> MEQCGAQAGGARCPNCLCCSRWGWCGTTSDFCGDGCQSQCSGCGPTPTPTPPSPSDGVGSIVPRDLFERLLLHRNDGACPARGFYTYEAFLAAAAAFPAFGGTGNTETRKREVAAFLGQTSH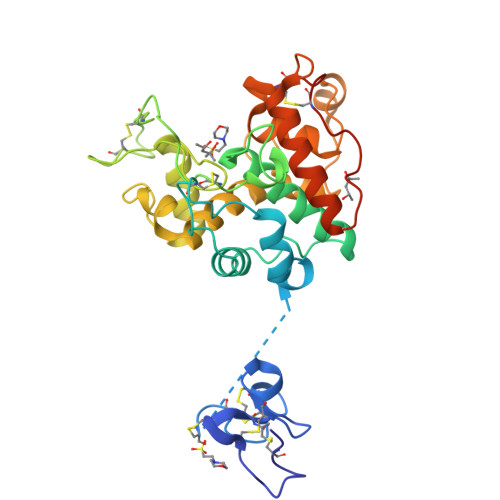ETTGGWPTAPDGPFSWGYCFKQEQNPPSDYCQPSPEWPCAPGRKYYGRGPIQLSFNFNYGPAGRAIGVDLLSNPDLVATDATVSFKTALWFWMTPQGNKPSSHDVITGRWAPSPADAAAGRAPGYGVITNIVNGGLECGHGPDDRVANRIGFYQRYCGAFGIGTGGNLDCYNQRPFNSGSSVGLAEQ>[2x]MKITVIGAGNVGATTAFRLAEKQLARELVLLDVVEGIPQGKALDMYESGPVGLFDTKVTGSNDYADTANSDIVVITAGLPRKPG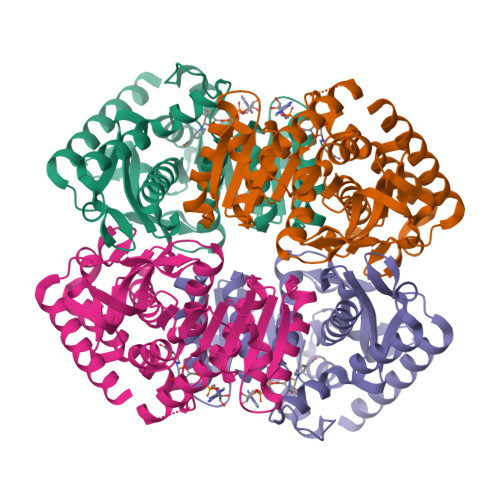MTREDLLSMNAGIVREVTGRIMEHSKNPIIVVVSNPLDIMTHVAWQKSGLPKERVIGMAGVLDSARFRSFIAMELGVSMQDVTACVLGGHGDAMVPVVKYTTVAGIPVADLISAERIAELVERTRTGGAEIVNHLKQGSAFYSPATSVVEMVESIVLDRKRVLTCAVSLDGQYGIDGTFVGVPVKLGKNGVEHIYEIKLDQSDLDLLQKSAKIVDENCKMLDASQG>MKKETIFSEVETANSKQLAVLKANFPQCFDKNGAFIQEKLLEIIRASEVELSKESYSLNWLGKSYARLLANLPPKTLLAEDKTHNQQEENKNSQHLLIKGDNLEVLKHMVNAYAEKVKMIYIDPPYNTGKDGFVYNDDRKFTPEQLSELAGIDLDEAKRILEFTTKGSSSHSAWLTFIYPRLYIARELMREDGTIFISIDHNEFSQLKLVCDEIFGEQNHVGDLVWKNATDNNPSNIAVEHEYIIVYTKNKEQLISEWKSNISDVKNLLVNIGEEFASKYTGNELQEKYTQWFREHRSELWPLDRYKYIDKDGIYTGSQSVHNPGKEGYRYDIIHPKTKKPCKQPLMGYRFPLDTMDRLLSEEKIIFGDDENKIIELKVYAKDYKQKLSSVIHLDGRVATNELKELFPEMTQPFTNAKTIKLVEDLISFACDGEGIVLDFFAGSGTTAHTVFNLNNKNKTSYQFITVQLDEPTKDKSDAMKHGYNTIFDLTKERLIRASKKNRDQGFKVYQLMPDFRAKDESELTLSNHTFFDDVVLTPEQYDTLLTTWCLYDGSLLTTPIEDVDLGGYKAHLCDGRLYLIAPNFTSEALKALLQKVDSDKDFAPNKVVFYGSNFESAKQMELNEALKSYANKKSIELDLVVRN[2x];> MSKGFTLEKNLPHQKAGVDAVMNVFVSATPHLTDNVAVRLLANPELKLSEQQYYNNIKNVQAFNGIAHSKDNHNAKSNIIDVSMETGTGKTYTYIKTIFDLNKSFGINKFIIIVPTLSIKAGTVNFLKSDALKEHFRDDYKRELRTYVVESQKNAGKNTKSYMPQAIHDFVEASNFNKKYIHVLVINSGMINSKSLTDTYDTGLLDNQFNTPVDALRAVKPFIIIDEPHRFPTGKKTWENIEKFNAQYIIRYGATFSEGYKNLVYRLTAVDAFNDDLVKGIDAYIEDIVGDGNANLKFVKSDGKEATFELNENNNKKSFKLAKGESLSKTHSAIHDLTLDALNKSTAVLSNGIELKIGSSINPYSYDQTLADNMMRKAVKEHFKLEKELLTQRPRIKPLTLFFIDDIEGYRDGNDISGSLKTKFEEYVLAEANELLKTEQDAFYKNYLEKTVTNISSVHGGYFSKDNSDKDDKIEQEINEILHDKELLLSLDNPRRFIFSKWTLREGWDNPNVFQICKLRSSGSTTSKLQEVGRGLRLPVNEYMCRVKDRNFTLKYYVDFTEKDFVDSLVKEVNESSFKERVPSKFTQELKEQIMAQYPELSSRALMNELFNDEIIDDNDNFKD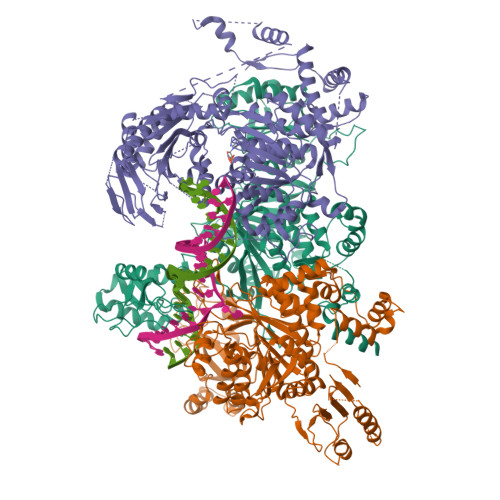SDAYSRLKSKYPAAFPIGVKPGKIKKATDGKRRTKMRVGKFSELKELWDLINQKAVIEYKINSESEFLSIFKSFMLEETERFTKSGVHTRIDKIYIHNDMAMSKSIVSDDDDFAKLNTMSYREFLDNLSQTIFVKHGTLHKVFCDIKDTINITEYLNIQTIRKIKSGFSKYLLNNSFNKFSLGYNLISGSIHPTKFTNADGNPLGEVLSSDLGVLQDNAKAPLDTYLFEEVFYDSELERRNITDREIQSVVVFSKIPKNSIKIPVAGGYTYSPDFAYVVKTAEGDYLNFIIETKNVDSKDSLRLEEKRKIEHAQALFNQISQSVKVEFRTQFANDDIYQLIKSALP>DFFRDEAERIMRDSPVIDGHNDLPWQLLDMFNNRLQDERANLTTLAGTHTNIPKLRAGFVGGQFWSVYTPCDTQNKDAVRRTLEQMDVVHRMCRMYPETFLYVTSSAGIRQAFREGKVASLIGVEGGHSIDSSLGVLRALYQLGMRYLTLTHSCNTPWADNWLVDTGDSEPQSQGLSPFGQRVVKELNRLGVLIDLAHVSVATMKATLQLSRAPVIFSHSSAYSVCASRRNVPDDVLRLVKQTDSLVMVNFYNNYISCTNKANLSQVADHLDHIKEVAGARAVGFGGDF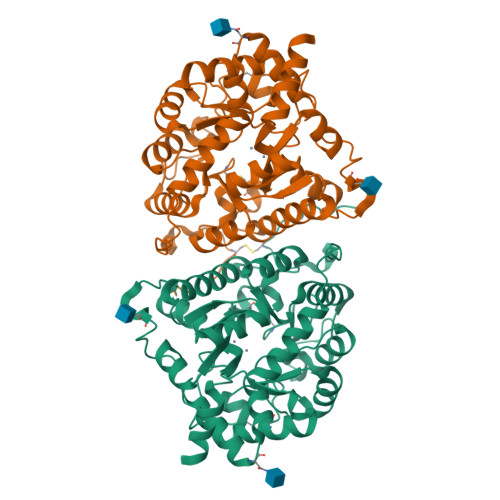DGVPRVPEGLEDVSKYPDLIAELLRRNWTEAEVKGALADNLLRVFEAVEQASNLTQAPEEEPIPLDQLGGSCRTHYGYSS[2x]> GEFELMEMILEEKDASDWIYRGEGGANLVLAYAGSSPLFVGKVIRIQKARRNDKAIKNSNGVVSVLTSDEQHLWRENNELISSPNKEVLEQRYVQNVIIPLLGPKHVDAGVRVSVSKEFLECVD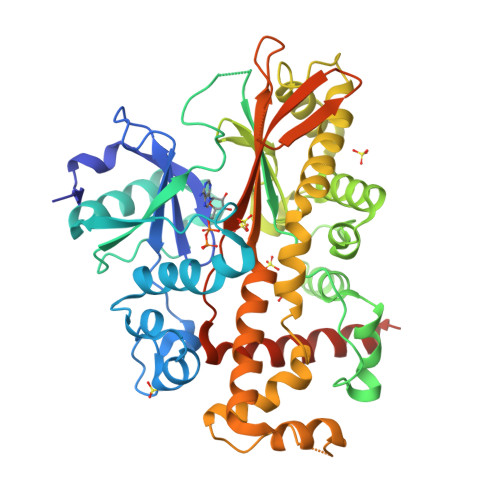KKVTKQRPLWRVNAANVDTSHDSALILNDHSLFSQGITSGGDCISVEIKPKCGFLPTSRFIGKENMLKTSVSRFKMHQLLKLEYIEISEESEYDPLDLFSGSKERVLEAIKALYSTPQNNFRVFLNGSLILGGSGESTGRTSPEIGYAFEDALKGFIQSEDGHRTECFLQLVSDAVYGSGVLDRLLEIQKLDKLDIEGAIHCYYDIINQPCPICKEGRPLEAELSLHALPLDESLKIVKEYLIAATAKDCSIMISFQSRNAWDSEPSGDYVSLKPTNQTFDYKVHFIDLSLKPLKRMESYYKLDKKIISFYNRKQKAENTAEQIGNSKPSHS Glutathione transferases (GSTs) constitute a widespread superfamily of enzymes notably involved in xenobiotic detoxification and/or in specialized metabolism. PtGSTU19 and 20, two paralogs sharing more than 91% sequence identity (95% of sequence similarity), would have diverged from a common ancestor of P. trichocarpa and P. yatungensis species. These enzymes display the distinctive glutathione (GSH)-conjugation and peroxidase activities against model substrates. PtGSTU19 and U20 have the same secondary structures as the known GSTU structures and show the canonical cytosolic GST fold.

The crystal structures of PtGSTU19 and 20 were solved in their apo form (U19 APO and U20 APO ) and in complex with GSH (U19 GSH and U20 GSH ). The H-site of PtGSTU19 has distinct properties. Nearly two-thirds of the helix α6 of U19APO (residues Val159 to Gly170) were refined in two conformations. The first conformation corresponds to the one found in U20APO/GSH/GS-PAP with Trp161 buried (ASA of 10 Å2) and a deep H-site. In the second conformation, Trp161 is more exposed to the solvent (ASA of 44 Å2), which reduces the depth of the pocket. In addition, the side chain of Tyr160 points in the direction of the assumed catalytic serine residue (Ser12). To our knowledge, this is the first time that this helix is observed in two conformations in the apo form and in one conformation in the GSH-bound form. Two-thirds of the α6 helix is flexible in PtGSTU19 while only one conformation is observed in PtGSTU20. The disorder of this α6 helix could explain why it was not possible to obtain crystallographic structures of PtGSTU19 in complex with flavonoids. In any case, this region (Glu34 to Lys51) is one of the regions with the highest B factors in PtGSTU19APO.

> MADVKLHGFWASPFSYRVIWALKLKGVEFEYIEEDLANKSELLLKYNPVYKQIPVFVHGGKPIAESLVILEYIEETWPENPLLPTDPYERAMARFWIQYGATKSAAFGALFRASGEELEKAAKEVVEVLRVLQEQGLGDKKFFGGDSINLVDISYGLFVYWLAAIEDIVGVKVLEPSTLPRLHAWAQNFIEVPLIKENHPDNDKLLLHMKGVREKMMNK>MPHSELSELPMPSPASEEVGALYDRFTALGAASLGENLHFGYWDSPDSQVPLAEATDRLTDMMAERLRIGAGSRVLDLGCGVGTPGVRIARLSGAH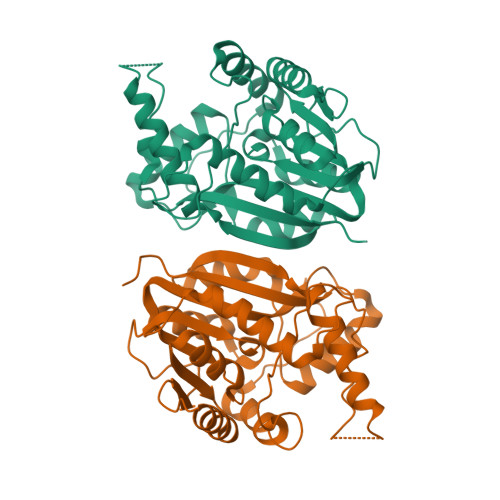VTGISVSHEQVVRANALAEEAGLADRARFQRADAMDLPFEDESFDAVIALESIIHMPDRAQVLAQVGRVLRPGGRLVLTDFFERAPLAPEGRAAVQRYLHDFMMTMVSAEAYPPLLRGAGLWLEEFLDISDQTLEKTFRLLSERINSSKQRLETQFGEEMVNQFDPGDLVGVKEFGYLLLVAQRPGKHHHHHH[2x]> ANNLGSKLLVGYWHNFDNGTGIIKLKDVSPKWDVINVSFGETGGDRSTVEFSPVYGTDADFKS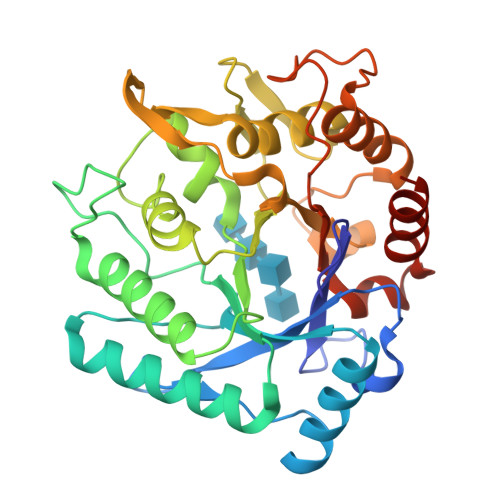DISYLKSKGKKVVLSIGGQNGVVLLPDNAAKDRFINSIQSLIDKYGFDGIDIDLGSGIYLNGNDTNFKNPTTPQIVNLISAIRTISDHYGPDFLLSMAPETAYVQGGYSAYGSIWGAYLPIIYGVKDKLTYIHVQHFNAGSGIGMDGNNYNQGTADYEVAMADMLLHGFPVGGNANNIFPALRSDQVMIGLPAAPAAAPSGGYISPTEMKKALNYIIKGVPFGGKYKLSNQSGYPAFRGLMSWSINWDAKNNFEFSNNYRTYFDGLSLQK>[2x]GSEFQNKNFRAPQSEAIGILYKLIETGSKHKNMYDHTEITTDSLLALLG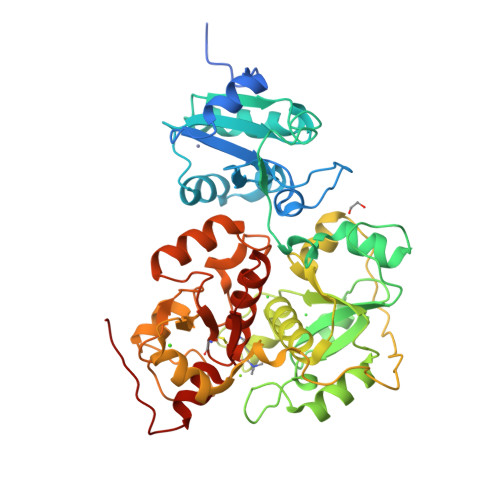SEKVKIIDVRSADAYNGWRMRGEVRGGHIKGAKSLPAKWLTDPEWLNIVRFKQIRPEDAIVLYGYTPEECEQTATRFKENGYNNVSVFHRFHPDWTGNDAFPMDRLEQYNRLVPAEWVNGLISGEEIPEYDNDTFIVCHAHYRNRDAYLSGHIPGATDMDTLALESPETWNRRTPEELKKALEEHGITASTTVVLYGKFMHPDNADEFPGSAAGHIGAIRLAFIMMYAGVEDVRVLNGGYQSWTDAGFAISKDDVPKTTVPEFGAPIPSRPEFAVDIDEAKEMLQSEDSDLVAVRSYPEYIGEVSGYNYIKKKGRIPGAIFAEAGSDAYHMENYRNHDHTTREYHEIEDIWAKSGIIPKKHLAFYCGTGWRGSEAWFNALLMGWPRVSVYDGGWFEWSNDPENPYETGVPK>GNNMYKLSENNHKSLLENLKRRGIIDDDDVYNTMLQVDRGKYIKEIPYIDTPVYISHGVTISAPHMHALSLKRLINVLKPGSRAIDVGSGSGYLTVCMAIKMNVLENKNSYVIGLERVKDLVNFSLENIKRDKPELLKIDNFKIIHKNIYQVN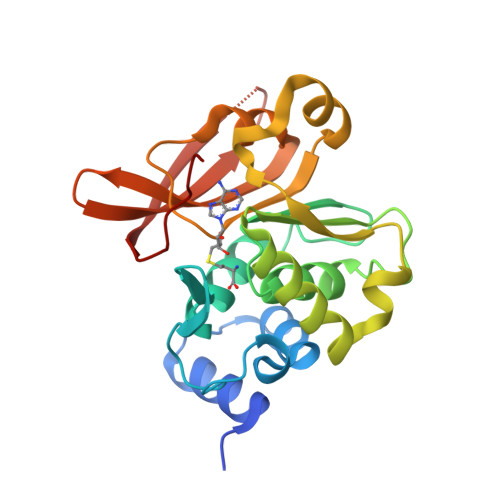EEEKKELGLFDAIHVGASASELPEILVDLLAENGKLIIPIEEDYTQVLYEITKKNGKIIKDRLFDVCFVSLKKN[2x]Coxsackievirus A9 (CVA9) belongs to the Enterovirus genus, species Enterovirus B (EV-B) in the family Picornaviridae. Like other picornaviruses, CVA9 has a small, ~30-nm-diameter, nonenveloped viral capsid. Its positive-sense single-stranded RNA genome is ~7,500 bases long and encodes 4 structural proteins (VP1 to 4) and 7 nonstructural proteins (2A to C and 3A to D). During cell entry, enterovirus capsids undergo conformational changes leading to expansion, formation of large pores, externalization of VP1 N termini, and loss of the lipid factor from VP1.

For CVA9 in DPBS, the addition of RNase gave lower fluorescence values, indicating that either nucleic acids were present in the CVA9 preparation or vRNA was released from a small percentage of the virions and was degraded by the RNase (black dotted line). Incubation of CVA9 in 0.01% fatty acid-free bovine serum albumin (faf-BSA) induced a fluorescent signal starting at 20 min and reaching its plateau at 40 min (Fig. 1B, red solid line). faf-BSA sequesters fatty acids from the virion. Addition of RNase in a parallel measurement showed only a slightly decreased fluorescence readout (red dotted line versus red solid line). This indicated that 0.01% faf-BSA in DPBS efficiently converted CVA9 into expanded particles and only a small fraction of virions dissociated, releasing their vRNA. Compared to the intact virions, the two cryo-EM reconstructions of CVA9 virions treated in two different ways, 0.01% faf-BSA or ion composition, yielded RNA-containing A-particles expanded by approximately 4% in diameter. In addition, these reconstructions revealed more flexibility in capsid proteins and no density for the lipid factor. The MS results indicated that there were only nonstoichiometric amounts of VP4 present and no VP4 could be modeled into the reconstructions. Further comparison of the two expanded particle reconstructions showed subtle differences between them. First, less of the VP1 N terminus was ordered in the ion-treated CVA9, where the first modeled residue was Ser60, compared to Lys54 in faf-BSA-treated CVA9. In contrast, the faf-BSA treatment of CVA9 generated more stable A-particles, as seen by the fluorescence assay and AF4. The CVA9 treatment with albumin induced expansion in the majority of the particles exposing the VP1 N termini in about 30 min, whereas most of the particles still contained vRNA. When virions were treated with faf-BSA, the lipid factor was bound more strongly by the albumin than by the capsid, causing the capsid to expand.

> GDVEEAIERAVVHVADTMRSGPSNSASVPALTAVETGHTSQVTPSDTMQTRHVKNYHSRSESTVENFLGRSACVYMEEYKTTDNDVNKKFVAWPINTKQMVQMRRKLEMFTYLRFDMEVTFVITSRQDPGTTLAQDMPVLTHQIMYVPPGGPIPAKVDDYAWQTSTNPSIFWTEGNAPARMSIPFISIGNAYSNFYDGWSNFDQRGSYGYNTLNNLGHIYVRHVSGSSPHPITSTIRVYFKPKHTRAWVPRPPRLCQYKKAFSVDFTPTPITDTRKDINTVTTVAQSRRRGDMSTLNTH;> SPTVEECGYSDRVRSITLGNSTITTQECANVVVGYGRWPTYLRDDEATAEDQPTQPDVATCRFYTLDSIKWEKGSVGWWWKFPEALSDMGLFGQNMQYHYLGRAGYTIHVQCNASKFHQGCLLVVCVPEAEMGGAVVGQAFSATAMANGDKAYEFTSATQSDQTKVQTAIHNAGMGVGVGNLTIYPHQWINLRTNNSATIVMPYINSVPMDNMFRHYNFTLMVIPFVKLDYADTASTYVPITVTVAPMCAEYNGLRLAQAQ;> GLPTMNTPGSTQFLTSDDFQSPCALPQFDVTPSMNIPGEVKNLMEIAEVDSVVPVNNVQDTTDQMEMFRIPVTINAPLQQQVFGLRLQPGLDSVFKHTLLGEILNYYAHWSGSMKLTFVFCGSAMATGKFLIAYSPPGANPPKTRKDAMLGTHIIWDIGLQSSCVLCVPWISQTHYRLVQQDEYTSAGYVTCWYQTGMIVPPGTPNSSSIMCFASACNDFSVRMLRDTPFISQDNKLQ> GSHMATDSLQPARIKDSGLTREQAEQVLRVALKHQDYQLQRPGVFIDGDLQDENGKPPHPGYYDFSLGYNDPKAGATEYWGLFSVSLNTGDTWEIN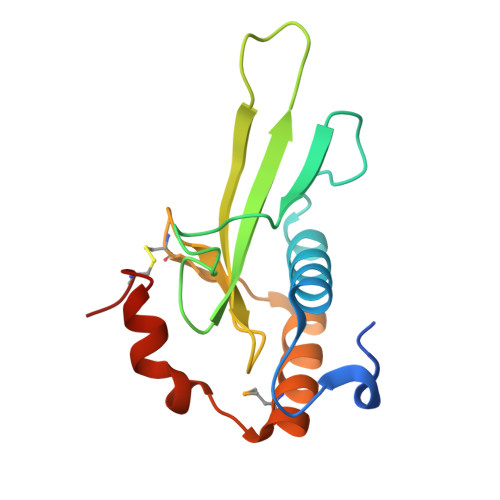SCKRLDGAELRALQRRVMARTGKSLADEKSQREGLGCEDQQ> MRVWVLAPHSLPPASFRPIFEARPPSSPTHSFHLLPTP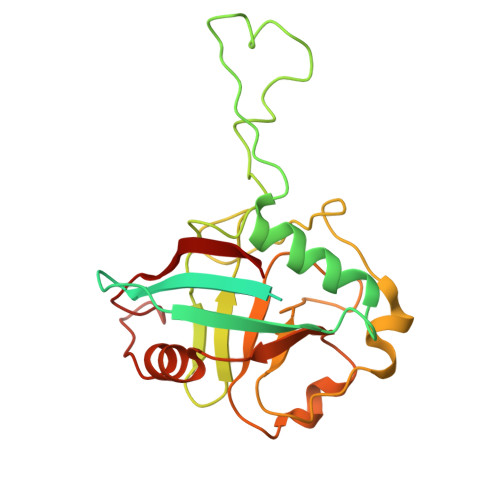IYLYITCTDAVDLYVCAVTSLLAEWTTTMFARSTIRWAAGAGHAFMDIAIGSQPPHRVTFELFTKRCPIASENFLKLCTGENVLPQVSSIDGIGEPSFRDQFLPQLTYRNTTVHRVCKGYLVQGGDIVSGQGTGQLSIYGESFDAPEEVKASKFDRMGLLGTAVSAPHLNGSQFFILTADKAPHLNGTCICFGRVVDGWTVVKAIEAIPLTAAGEPAERVVVVECGKL>[2x]MVSRYVPDMGDLIWVDF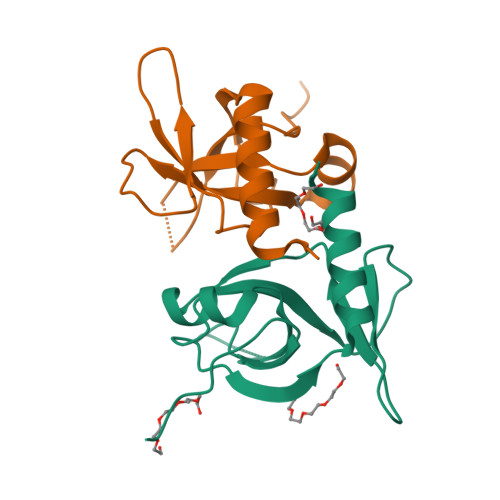DPTKGSEQAGHRPAVVLSPFMYNNKTGMCLCVPCTTQSKGYPFEVVLSGQERDGVALADQVKSIAWRARGATKKGTVAPEELQLIKAKINVLIGHHHHHH> MAIITPALISALKTSFQKHFQDALATAPST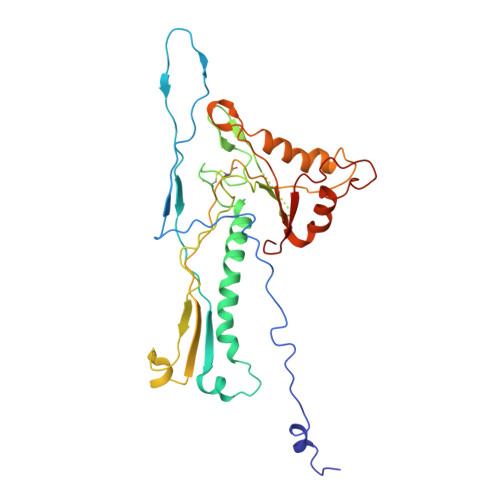YLQVATVIPSTTASNTYGWLGQFPKLREWIGQRVIKDMAAQGYQITNKLFESTVGVKRTDIEDDNLGVYGPLMQEMGRAAGAHPDELVFALLKAGNANLCYDGQNFFDTDHPVYPNVDGTGTATTVSNLFAPAADPGAAWYLLDTSRSLKPLIYQERMKPSFTSMTKEDDEQVFMADEYRYGVRSRCNVGFGFWQLAAMSTEELNQVNFEKVYDAMRNQKADGGRPLDIRPNLLVVPTTLRSKAKEVVGVQRLANGADNPNFELVQVLDTAWLN>[2x]CGC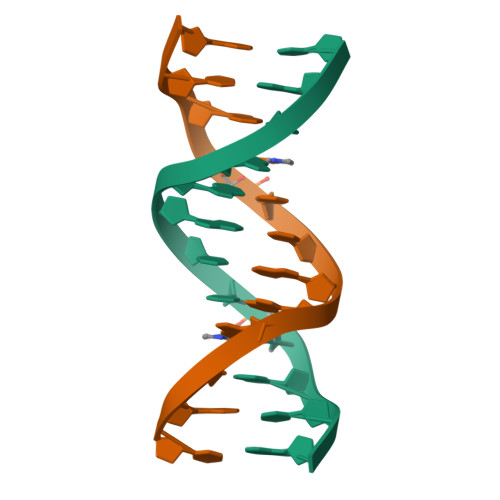GAATTAGCG> MDTASCPVTTEGDYVWKISEFYGRKPEGTYYNSLGFNIKATNGGTLDFTCSAQADKLED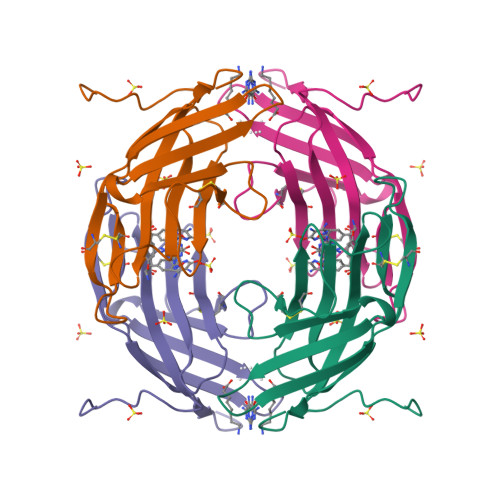HKWYSCGENSFMDFSFDSDRSGLLLKQKVSDDITYVATATLPNYCRAGGNGPKDFVCQGVADAYITLVTLPKSS> MGPLSRDAWAQRLGAFRASPSAFMAGPEGEDLGRDLLSDLRSEKLSEQTKVSLLALSMEYPAQLWPDASAAEVAATSLLDTLVLLPPRPSALRRPLLLAATTALAAGGALGPTSGASCRLLPLLLGLAAGSDLGRGFVPASEQRPLQATACECLRELESCKPGLLGGSLGLLRGLLGQEGPVQPLSLLLALALRNTLVLQSRVGAGLGGLLTDKVSPTGGGPWDWTLVEEGDGRLQPQAPSWPAAEEGEGERSLTAREHSPEEARELRAAVIQLLDTSYLLTPVAQAQLLW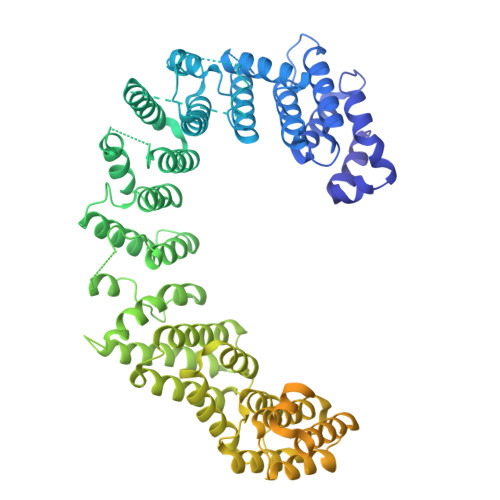LLGWALRGLQGQPPALFKPQLVRLLGTAQLTLLHAMLALKAAFGEALFTAQDEALLLRRLTLAAQHPALPPPTHLFYLHCVLSFPENWPLGPEGEEAAPLLLGPQLCRGLLPSLLHDPMALLARLHLLCLLCAEEEEEEKGQLPSPRHYLEELLAGLRQRAALDGGPRALATLCFQASYLVACCLAGQPTVLTPLIHGLAQLYQARPMLAPHFVDLLDQVDSELREPLKVVLRQVVVSRPGRDEALCWHLQMLAKVADGDAQSATLNFLQAAAAHCTNWDLQQGLLRVCRALLRAGVRGGLVDLLQVLARQLEDPDGRDHARLYYILLAHLAAPKLGVALGPSLAAPALASSLVAENQGFVAALMVQEAPALVRLSLGSHRVKGPLPVLKLQPEALEPIYSLELRFRVEGQLYAPLEAVHVPCLCPGRPARPLLLPLQPRCPAPARLDVHALYTTSTGLTCHAHLPPLFVNFADLFLPFPQPPEGAGLGFFEELWDSCLPEGAESRVWCPLGPQGLEGLVSRHLEPFVVVAQPPTSYCVAIHLPPDSKLLLRLEAALADGVPVALRTDDWAVLPLAGDYLRGLAAAV> VTAFDPTDADVRRDPYPSYHWLLRHDPVHRGAHRVWYVSRFADVRAVLGDERFARTGIRRFWTDLVGPGLLAEIVGDIILFQDEPDHGRLRGVVGPAFSPSALRRLEPVIAGTVDDLLRPALARGAMDVVDELAYPLALRAVLGLLGLPAADWGAVGRWSRDVGRTLDRGASAEDMRRGHAAIAEFA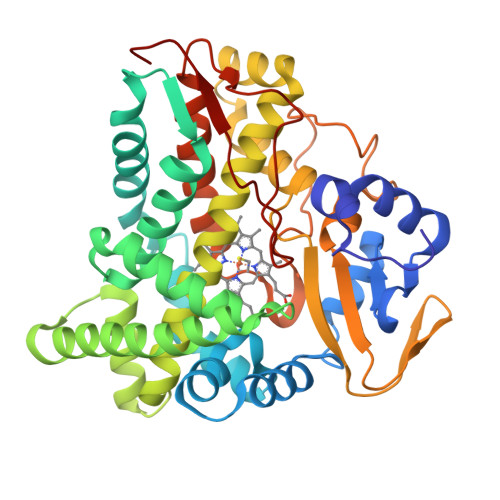DYVERALARRRREGGEDLLALMLDAHDRGLMSRNEIVSTVVTFIFTGHETVASQVGNAVLSLLAHPDQLDLLRRRPDLLAQAVEECLRYDPSVQSNTRQLDVDVELRGRRLRRDDVVVVLAGAANRDPRRYDRPDDFDIERDPVPSMSFGAGMRYCLGSYLARTQLRAAVAALARLPGLRLGCASDALAYQPRTMFRGLASLPIAFTPGG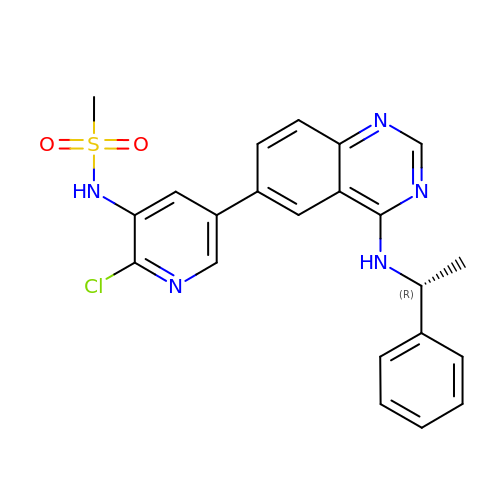N-[(5P)-2-chloro-5-(4-{[(1R)-1-phenylethyl]amino}quinazolin-6-yl)pyridin-3-yl]methanesulfonamide | C22 H20 Cl N5 O2 S | LPJIZDSOUGHTNB-CQSZACIVSA-N> MMVFQSFILGNLVSLCMKIINSVVVVGLYYGFLTTFSIGPSYLFLLRARVMDEGEEGTEKKVSATTGFIAGQLMMFISIYYAPLHLALGRPHTITVLALPYLLFHFFWNN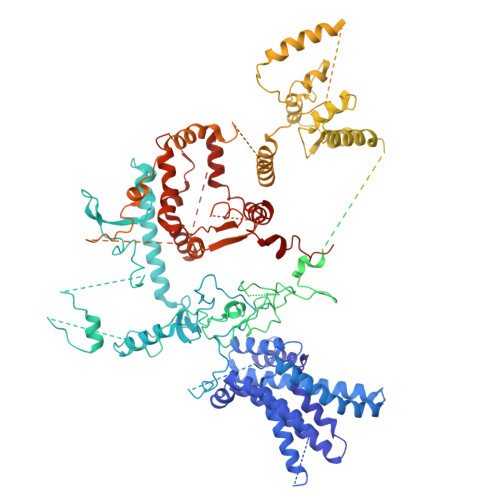HKHFFDYGSTTRNEMRNLRIQCVFLNNLIFQLFNHFILPSSMLARLVNIYMFRCNNKMLFVTSSFVGWLIGHILFMKWVGLVLVWIQQNNSIRSNVVIRSNKYKFLVSELRNSMARIFSILLFITCVYYLGRIPSPIFTKKLKGTSETGGTKQDQEVSTEEAPFPSLFSEEGEDLDKIDEMEEIRVNGKDKINKDDEFHVRTYYNYKTVSENLYGNKENSNLEFFKIKKKEDHFLWFEKPFVTLVFDYKRWNRPNRYIKNDKIENIVRNEMSQYFFYTCQSDGKERISFTYPPNLSTFFEMIQKRIPSFTKEKKTFDQVSTYWSLIHEEKRENLKKEFLNRIEALDKEWSVENILEKTTRFCYNEAKKEYLPKIYDPFLHGISRGRIKKLPPFQIITETYRKNNLGGSWINKIHGLLLKINYKKFEQTIEKFNRKSLSIEKKLSFFSEPQQEEKINSEEEIKTFKFLFDIVRTDSNDQTLIKNFMDFPEINKKVPRWSYKLISELEELEGENEENVPMEPGIRSRKAKRVVVFTDKEPHGEIYTNLKDNQNSDQNDEMALIRYSQQSDFRREIIKGSMRSQRRKTVIWEFFQAKVHSPLFFDRIDKLFFFSFDIWGLKKKIIKNFIWKKKIDKKEEEQSKREETRRIEIAETWDSFLFAQIIRGSLLVTQSILRKYIILPLLIIIKNSVRMLLFQFPEWSQDLKDWKREMHVKCTYNGVQLSETEFPRNWLTDGIQIKILFPFYLKPWHKSKFQASQKARLKKTKDKGEKNDFCFLTVWGMETELPFGSAQRKPSFFEPISKELKKRIKKLKKKSFVVLKIFKERAPIFLKVAKETKNWILKNFIFIKGISKRNLIPLFGPREIYELNEPKKDSIISNQMIHELSVQNKSLEWTNSSLSEKKIKNLIDRKKTIRNQIEEISKEKQNLTNSCTKLRYDSKIIESSKKIWQTFKRKNTRLIRKSIFFFKFCIEQMSIAIFLGIINIPRITTQLFFESTKKILDKYIYKNEENGEKKKNTLYFISTIKNLISNKKKMSYDLCSLSQAYVFYKLSQIKVSNFCKLKAVLEYNICITSFFVKNKIKVFFQEHGIFHYELKNKTFLNSEVNQWKNWLRSQYQYNLPQISWARLVTQNWKNKINKDSLVLNPSLTKEDSYEKKKFDNYKKQKFFEADSLLNPKHNVKKDSIYNLFCYKSIHSTEKNFDMSIGIALDNCLVSSFLEKYNIRGMGEIRHRKYLDWRILNFWFTKKVTIEPWVDTKSKKKYINTKVQNYQKIDKITQTDLANKKRNFFDWMGMNEEILNQRITNFEFFFFPEFFLFSSTYKMKPWVIPIKLLLLNFNENINVNKKIIRKKKGFIPSNEKESLRFYNLNKEEKESAGQVELESDKETKRNPEAARLNQEKNIEENFAESTIKKRKNKKQYKSNTEAELDLFLTRYSRFQLRWNCFFNQKILNNVKVYCLLVRLNNPNEIAVSSIERGEMSLDILMIEKNFTFAKLMKKGILIIEPVRLSVQNDGQLIIYRTIGISLVHKNKHKISKRYKKKSYINKKFFEKSITKYQNKTVNKKKNNYDFFVPEKILSPKRRREFRILICFNLKKKNARDTNSRFDKNIQNLTTVLHKKKDLDLDKDKNNLINLKSFLWPNFKLEDLACMNRYWFNTTNGNHFSMIRIRMYTRFPIP METHYL 2-[4-METHOXY-6-METHYL-1,3,5-TRAZIN-2-YL(METHYL)CARBAMOYLSULFAMOYL]BENZOATE 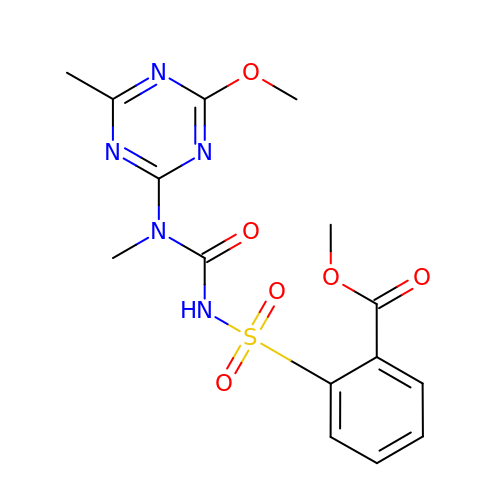| C15 H17 N5 O6 S | VLCQZHSMCYCDJL-UHFFFAOYSA-N>MKQKVHSVSYLAKAEFEYKNGVYDLVALPTGAEVIKISLEVVGLPTAGHVSVGFKDESKKNYSSILTLPVNETSGVVTKDYTVKSDKIVAAEVKDALAEGSDGRPVKCVLRALYFL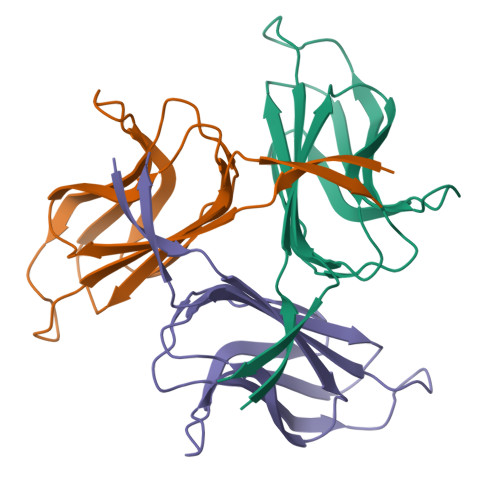PSVIEVEY[3x]> MKILVAVKQTAALEEDFEIREDGMDVDEDFMMYDLNEWDDFSLEEAMKIKESSDTDVEVVVVSVGPDRVDESLRKCLAKGADRAVRVWDDAAEGSDAIVVGRILTEVIKKEAPDMVFAGVQSSDQAYASTGISVASYLNWPHAAVVAD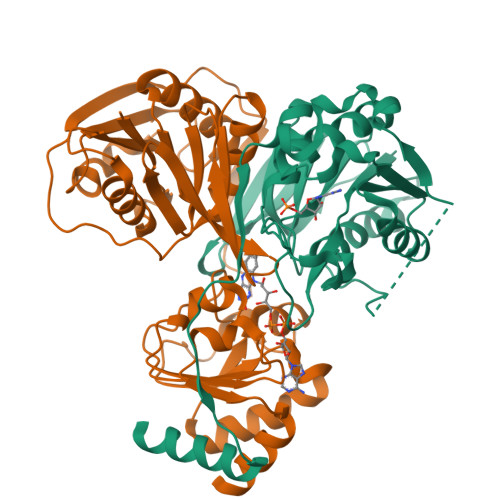LQYKPGDNKAVIRRELEGGMLQEVEINCPAVLTIQLGINKPRYASLRGIKQAATKPIEEVSLADIGLSANDVGAAQSMSRVRRMYIPEKGRATMIEGTISEQAAKIIQIINEFKGA;> SKILVIAEHRRNDLRPVSLELIGAANGLKKSGEDKVVVAVIGSQADAFVPALSVNGVDELVVVKGSSIDFDPDVFEASVSALIAAHNPSVVLLPHSVDSLGYASSLASKTGYGFATDVYIVEYQGDELVATRGGYNQKVNVEVDFPGKSTVVLTIRPSVFKPLEGAGSPVVSNVDAPSVQSRSQNKDYVEVGGGNDIDITTVDFIMSIGRGIGEETNVEQFRELADEAGATLCCSRPIADAGWLPKSRQVGQSGKVVGSCKLYVAMGISGSIQHMAGMKHVPTIIAVNTDPGASIFTIAKYGIVADIFDIEEELKAQLAA> VTGTNKVGTGKGVLGDTKSLNTTLSGSSYYLQDNTRGATIFTYDAKNRSTLPGTLWADADNVFNAAYDAAAVDAHYYAGKTYDY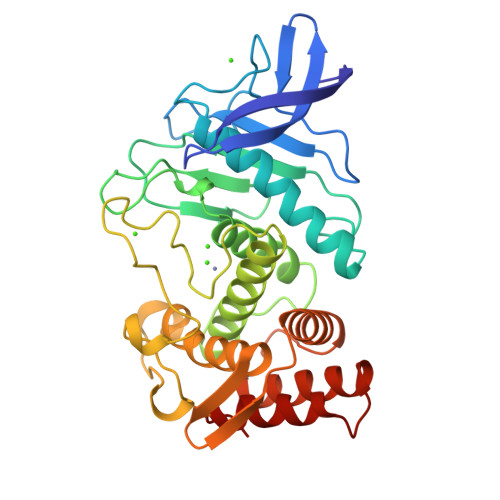YKATFNRNSINDAGAPLKSTVHYGSNYNNAFWNGSQMVYGDGDGVTFTSLSGGIDVIGHSLTHAVTENSSNLIYQNESGALNEAISDIFGTLVEFYDNRNPDWEIGEDIYTPGKAGDALRSMSDPTKYGDPDHYSKRYTGSSDNGGVHTNSGIINKQAYLLANGGTHYGVTVTGIGKDKLGAIYYRANTQYFTQSTTFSQARAGAVQAAADLYGANSAEVAAVKQSFSAVGVN> YIKANDINFGTRSVHDCRERTGIQRDVKVRADIPFETDDGPNQVLRVTWSNALNVDRFDPLPIVTVPG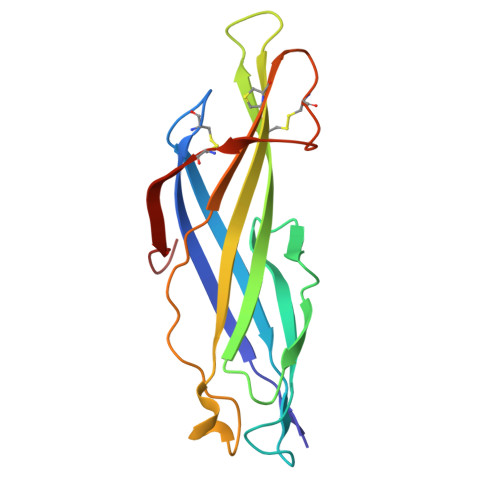NAASTTITAIHDFCLMNPTTSPPTRCLYQLRQPFTLGFDRTRMHNNIYLTPPNPQRPTMHEVCIRADECPAGRVFLECSTRTYGAIPRGE> VIGGNECDINEHRFLVAFFNTTGFFCGG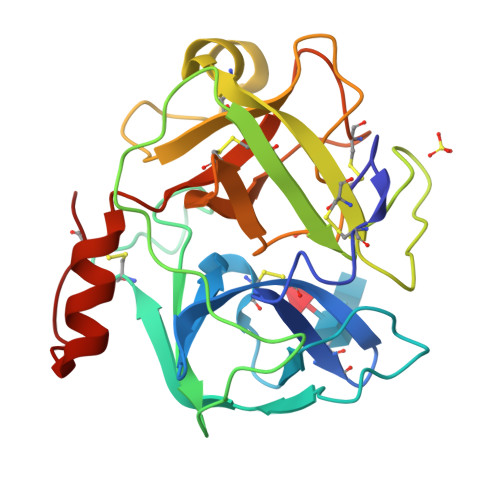TLINPEWVVTAAHCDSTDFQMQLGVHSKKVLNEDEQTRNPKEKFICPNKNNNEVLDKDIMLIKLDKPISNSKHIAPLSLPSSPPSVGSVCRIMGWGSITPVKETFPDVPYCANINLLDHAVCQAGYPELLAEYRTLCAGIVQGGKDTCGGDSGGPLICNGQFQGIVSYGAHPCGQGPKPGIYTNVFDYTDWIQRNIAGNTDATCPP>[2x]FACKTANGTAIPIGGGSANVYVNLAPVVNVGQNLVVDLSTQIFCHNDYP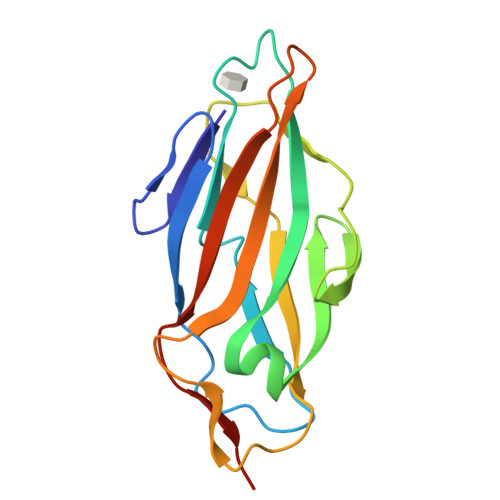ETITDYVTLQRGSAYGGVLSNFSGTVKYSGSSYPFPTTSETPRVVYNSRTDKPWPVALYLTPVSSAGGVAIKAGSLIAVLILRQTNNYNSDDFQFVWNIYANNDVVVPTHHHHHH>MGYTVAVVGATGAVGAQMIKMLEESTLPIDKIRYLASARSAGKSLKFKDQDITIEETTETAFEGVDIALFSAGSSTSAKYAPYAVKAGVVVVDNTSYFRQNPDVPLVVPEVNAHALDAHNGIIACPNCSTIQMMVALEPVRQKWGLDRIIVSTYQAVSGAGMGAILETQRELREVLNDGVKPCDLHAEILPSGGDKKHYPIAFNALPQIDVFTDNDYTYEEMKMTKETKKIMEDDSIAVSATCVRIPVLSAHSESVYIETKEVA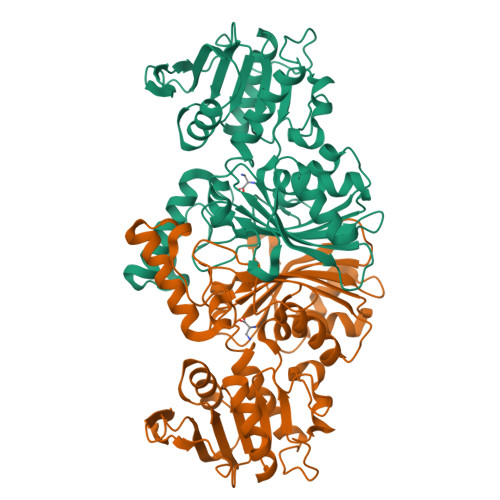PIEEVKAAIAAFPGAVLEDDVAHQIYPQAINAVGSRDTFVGRIRKDLDAEKGIHMWVVSDNLLKGAAWNSVQIAETLHERGLVRPTAELKFELKLEHHHHHH[4x]>GDHGMGFLSGKRILVTGVASKLSIAYGIAQAMHREGAELAFTYQNDKLKGRVEEFAAQLGSDIVLQCDVAEDASIDTMFAELGKVWPKFDGFVHSIGFAPGDQLDGDYVNAVTREGFKIAHDISSYSF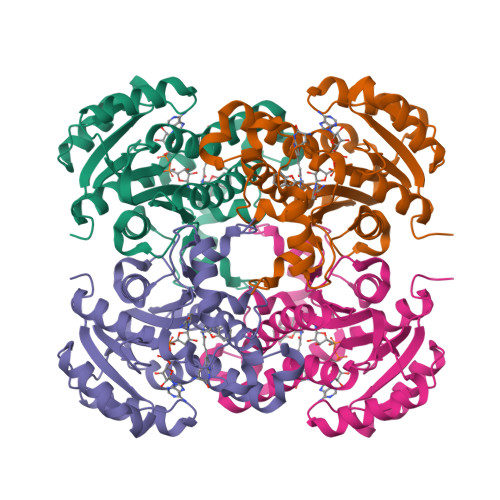VAMAKACRSMLNPGSALLTLSYLGAERAIPNYNVMGLAKASLEANVRYMANAMGPEGVRVNAISAGPIRTLAASGIKDFRKMLAHCEAVTPIRRTVTIEDVGNSAAFLCSDLSAGISGEVVHVDGGFSIAAMNELELK[2x]>[2x]MMKPEDVIKEQCARAKVVAELWHGFTGGAPKAALENLVVEFNKAQQGRCVRPVPQGGYRDLSTKIKAAFAAGKVPTMAQAFENNIALYLEAKALLPIESLGVKLQGVNLTFLNAVRFGGVVYGVPFNKSIQVLYYNKDLLKKHGVPVPATLEEFVAAAKKLSRAEGGPVYWFQPDASTFAYFFFN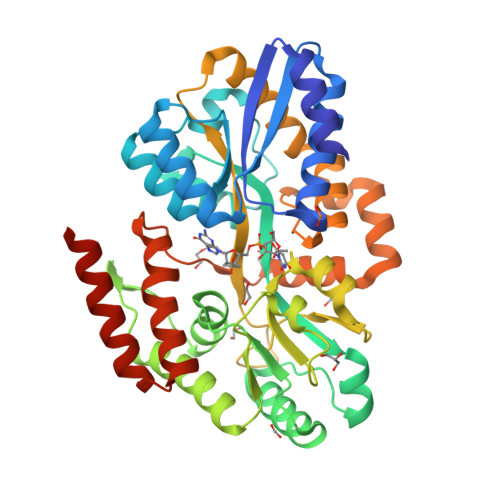LGGSYLKDGKLVLNSKEAVEALTLLQNGVKEGWAKPITSGYINQNLGSGPYAFSVDASAGYTYYLRAAKFDLGVATLPGRTKGQPGYGLVQGTNLVVFRQASKEEQAVAKDFLEFVLSPRAQAVFATATGYVPVTEGALKDPVYQAYAAENPDYATIVRQSRYAKFEPALAEWEQIRFDILGQAIKEAILNKADPKAALDRAQKLAEDLLSSRTRHHHHHH> MEKKKYTAPQLAKVGEFKEAT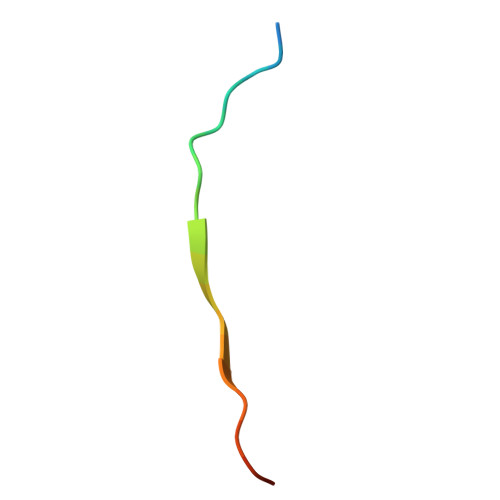G>MKHDYTNPPWNAKVPVQRAMQWMPISQKAGAAWGVDPQLITAIIAIESGGNPNAVSKSNAIGLMQLKASTSGRDVYRRMGWSGEPTTSELKNPERNISMGAAYLNILETGPLAGIEDPKVLQYALVVSYANGAGALLRTFSSDRKKAISKINDLDADEFLEHVARNHPAPQAPRFIYKLEQAL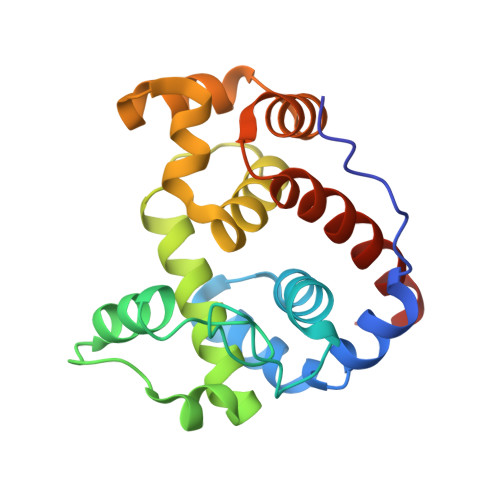DAMLEHHHHHH[2x]>GRMRIQEQSGARDKMVIGAGGLEDYIDKAMDDVAPNLKALVGAKLGARLISLAGGLKELAMLPSSTIQVLGAEKALFRHLRTGAKPPKHGVIYQYPAINRSPWWQRGKIARALAGKLAIAARVDYFSGEYIAEELKKELEARIKEIKEKYPRPPKRRKEERKGRK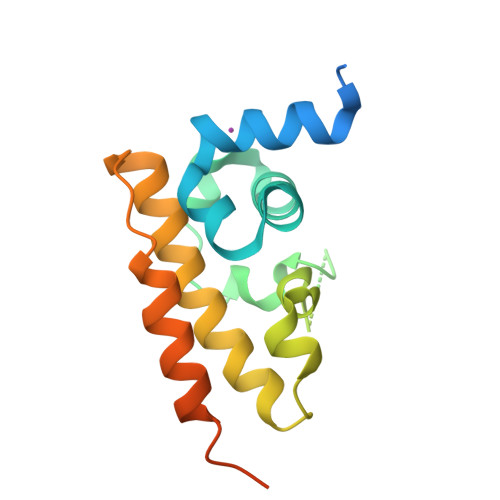PWKE[2x]>[3x]MVDWELMKKIIESPGVSGYEHLGIRDLVVDILKDVADEVKIDKLGNVIAHFKGSAPKVMVAAHMDKIGLMVNHIDKDGYLRVVPIGGVLPETLIAQKIRFFTEKGERYGVVGVLPPHLRREAKDQGGKIDWDSIIVDVGASSREEAEEMGFRIGTIGEFAPNFTRLSEHRFATPYLDDRICLYAMIEAARQLGEHEADIYIVASVQEEIGLRGARVASFAIDP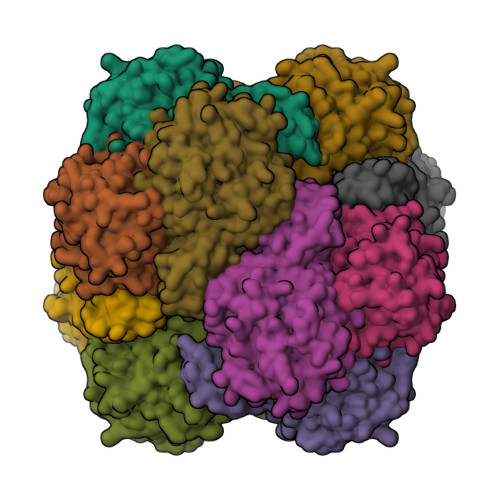EVGIAMDVTFAKQPNDKGKIVPELGKGPVMDVGPNINPKLRQFADEVAKKYEIPLQVEPSPRPTGTDANVMQINREGVATAVLSIPIRYMHSQVELADARDVDNTIKLAKALLEELKPMDFTP>[6x]MENGYTYEDYKNTAEWLLSHTKHRPQVAIICGSGLGGLTDKLTQAQIFDYGEIPNFPRSTVPGHAGRLVFGFLNGRACVMMQGRFHMYEGYPLWKVTFPVRVFHLLGVDTLVVTNAAGGLNPKFEVGDIMLIRDHINLPG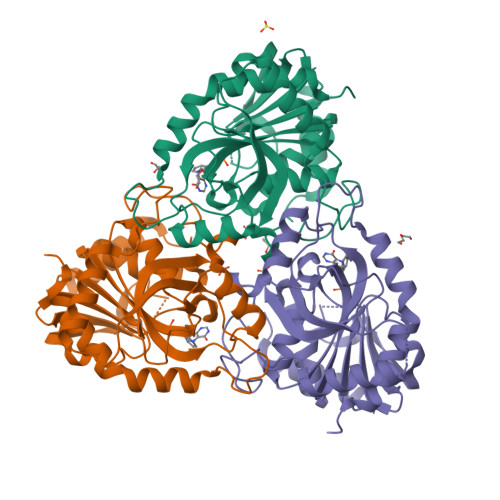FSGQNPLRGPNDERFGDRFPAMSDAYDRTMRQRALSTWKQMGEQRELQEGTYVMVAGPSFETVAECRVLQKLGADAVGMSTVPEVIVARHCGLRVFGFSLITNKVIMDYESLEKANHEEVLAAGKQAAQKLEQFVSILMASIPLPDKAS>[2x]MGHDIDQVAPLLREPANFQLRTNCDPHEDNFGLRAHGPLVRIVGESSTQLGRDFVW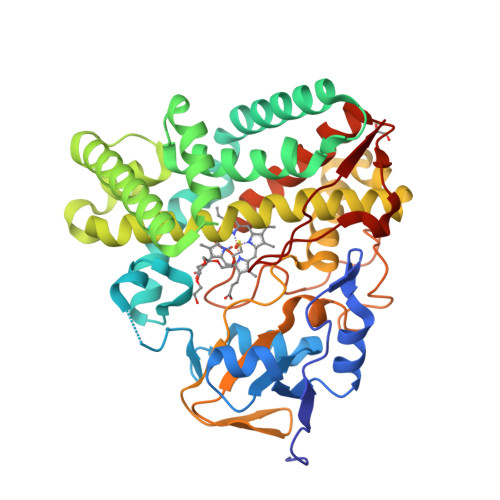QAHGYEVVRRILGDHEHFTTRPQFTQSKSGAHVEAQFVGQISTYDPPEHTRLRKMLTPEFTVRRIRRMEPAIQSLIDDRLDLLEAEGPSADLQGLFADPVGAHALCELLGIPRDDQREFVRRIRRNADLSRGLKARAADSAAFNRYLDNLLARQRADPDDGLLGMIVRDHGDNVTDEELKGLCTALILGGVETVAGMIGFGVLALLDNPGQIELLFESPEKAERVVNELVRYLSPVQAPNPRLAIKDVVIDGQLIKAGDYVLCSILMANRDEALTPDPDVLDANRAAVSDVGFGHGIHYCVGAALARSMLRMAYQTLWRRFPGLRLAVPIEEVKYRSAFVDCPDQVPVTW>[2x]KPKFFYIKSELNGKVLDI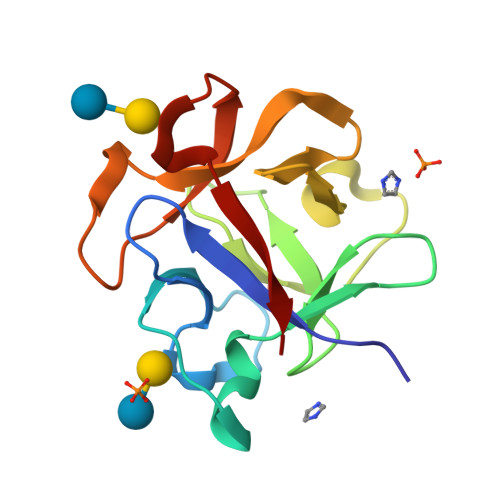EGQNPAPGSKIITWDQKKGPTAVNQLWYTDQQGVIRSKLNDFAIDASHEQIETQPFDPNNPKRAWIVSGNTIAQLSDRDIVLDIIKSDKEAGAHICAWKQHGGPNQKFIIESE> GGGUCAGGC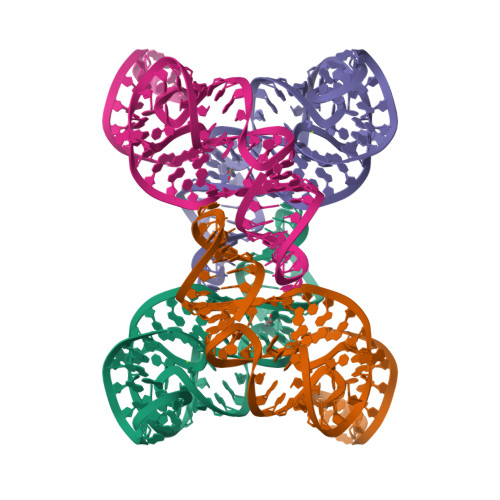CGGCGAAAGUCGCCACAGUUUGGGGAAAGCUGUGCAGCCUGUAACCCCCCCACGAAAGUGGG> GSSSGQSNNNSDTCAEFRIKYVGAIEKLKLSEGKGLEGPLDLINYIDVAQQDGKLPFVPPEEEFIMGVSKYGIKVSTSDQYDV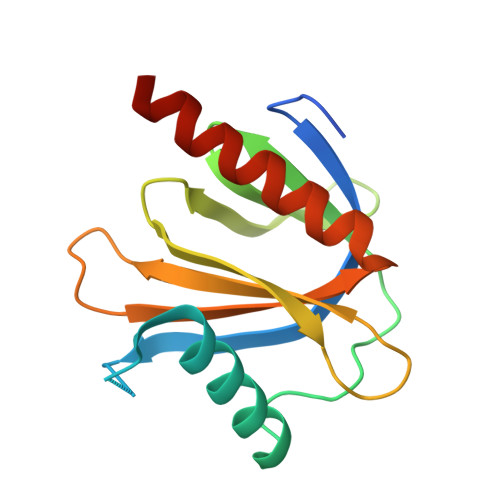LHRHALYLIIRMVCYDDGLGAGKSLLALKTTDASNEEYSLWVYQCNSLEQAQAICKVLSTAFDSVLTSEKP>[6x]MAMGDKAKLYRNISQRCLRRGSPEEALRYLKEWARHEKNDPEPLYQMGIALANLGD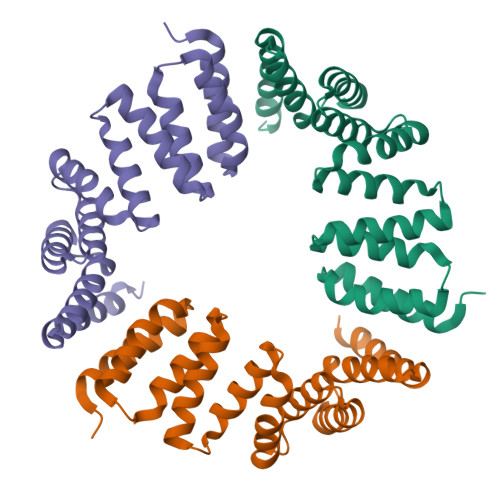YQRAVTVFDKVLKLRPNHFMASYRKGAVLLKIKQYKLALPVLEAVVAAAPADARAYYLLGLAYDGDEQLEKGIEAMQKAVDLDPEEIKYHQHLGFMNVRKDDHKTAAEHFTKVMELERSQDSDEEELALVPRGSSAHHHHHHHHHH> SNAQVNPSEEIFIGVAWPFASLDDLFAEGLELAVQEINEQGGVQGRKLSLVKADDEAELEKGLAIAQAFADNAGIQAVIGHRNSFISIPAASIYDQAGLVMLSPASTSPDLTDHGYIHVFRNIPSDQEIARQLAIYLAEQGHERMVIYYTDDSYGNGLANAFEDYARAQGITIVDRFNYYGNLKDLERLYDKWQAFGMDGIFIAKTATGGGTEFLVDAKSVGIEVPLIAGNSWDALSLTEDIENIGMTAEGLLVGSFFNPQRPDSRTQDFVEAFRREYGQPPTSYAAAGYDAVILLAEALEKSDLTHPATLAQGLRDLGPWEGVMGMHRFDGRGDDIGDLVVLKKMKDGR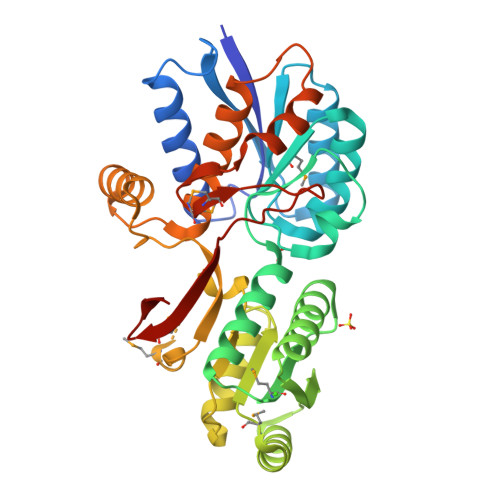FEYLGH>[2x]GSSGSSGMQAGKPILYSYFRSSCSWRVRIALALKGIDYEIVPINLIKDGGQQFTEEFQTLNPMKQVPALKIDGITIVQSLAIMEYLEETRPIPRLLPQDPQKRAIVRMISDLIA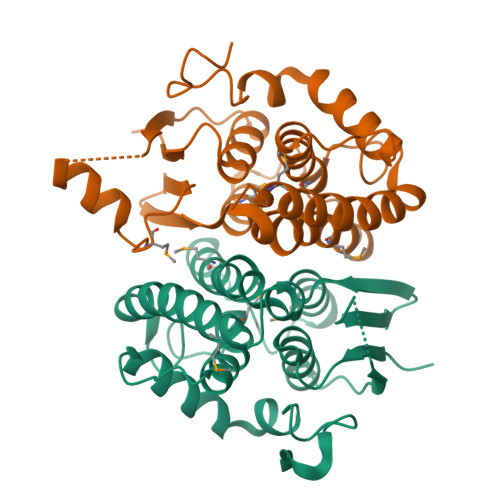SGIQPLQNLSVLKQVGQENQMQWAQKVITSGFNALEKILQSTAGKYCVGDEVSMADVCLVPQVANAERFKVDLSPYPTISHINKELLALEVFQVSHPRRQPDTPAELRT>GMISYLKKAEKTPQTETATAQKVVTEMLAEIQARGKDAVRQYAKQLDGWSGDIVLTPDQIREQTKDVPAGVRADIDFAIRQVTDFALAQRESLKEFSVELHPGVTAGQRVLPVNVVGCYAPAGRYAHIASAYMGVATAKAAGVKTVVACSSPFRGQGIHPHVLYAFQAAGADVIMALGGVQAIASMAYGLFTGKPADVVVGPGNKFVAEAKRSLYGQVGIDVFAGPSEVAVIADETADPAIVASDLVGQAEHGHESPAWLFTTSRDLADRVMALVPELIAKLPPTARDAATAAWRDYGEVILCGTREEVVEISDRYASEHLEVHTADLDWWLANLTCYGSLFLGEETTVAFGDKTSGPNHVLPTKGAARYSGGLSVHKFMKTLTWQQMTREATRQIGQVTARISRLEGMEAHARTADDRMAKYFPNASFEMGTPVEV[2x]

Here, we study DHPS-3-dehydrogenase from Cupriavidus pinatubonensis (CpHpsN), a bacterium capable of utilizing DHPS as a sole carbon source. Kinetic analysis of CpHpsN reveals a strict preference for R-DHPS, catalyzing its 4-electron oxidation to R-SL, with high specificity for NAD+ over NADP+. CpHpsN forms a domain-swapped tight dimer with 28% of surface area buried at the dimer interface, with the interface featuring extensive hydrophobic and hydrogen-bond interactions. Domain 4 lies at the C-terminus and contributes to the active site and is also involved in dimerization through a metal binding site. Coordination of Zn2+ involves three residues from one monomer and one residue (His411*; * denotes the other monomer in the dimer) from the other monomer (Fig. 5 and S7†), showing that the enzyme forms an obligate dimer.

Initially, the protein crystallized as the CpHpsN·Zn2+ complex in space group P212121 and the 3D structure was solved and refined to 1.94 Å resolution. CpHpsN structures in both space groups contain a dimer in the asymmetric unit. Comparison of the CpHpsN·Zn2+ and CpHpsN·Zn2+·NADH·R-SL structures reveals rearrangement in the octahedral coordination environment at the zinc center. In the CpHpsN·Zn2+ structure, Zn2+ is coordinated by four amino acid residues: three histidine residues (His126, His251 and His411*) and Gln248, and the remaining two equatorial sites (#3 and #6) were modelled as water (Fig. 5a and S7a†). Analysis of the interfaces using the Protein Interfaces, Surfaces and Assemblies interactive tool25 indicates that the CpHpsN·Zn2+·NADH·R-SL complex forms a more compact dimer versus CpHpsN·Zn2+, with the increased buried surface area from 9620 to 13 250 Å2 and decrease in ΔGdiss from 84.1 to 98.7 kcal mol−1. The root-mean square deviation of the CpHpsN·Zn2+ and CpHpsN·Zn2+·NADH·R-SL structures is 2.0 Å over 407 common Cα positions. In the Ramachandran plot of the CpHpsN·Zn2+ structure, Asp352 is placed in the right-handed α helix region, while in the CpHpsN·Zn2+·NADH·R-SL structure this residue lies in the β-sheet region, demonstrating a significant difference in the loop conformation near the active site. In a similar manner, Ala121 in the connecting loop (residues 120–128), which is placed in the left-handed α-helix region in the CpHpsN·Zn2+ structure, moves to the β-sheet region in the CpHpsN·Zn2+·NADH·R-SL structure.>MKTPEDCTGLADIREAIDRIDLD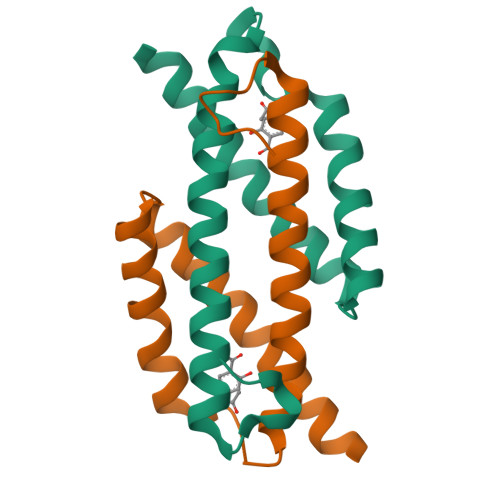IVQALGRRMDYVKAASRFEASEAAIPAPERVAAMLPERARWAEENGLDAPFVEGLFAQIIHWYIAEQIKYWRQTRGAA[2x]> MGSSHHHHHHSQDPMEIPLSSGNVNTPDVRSSGILYINIYPIVNYPETIKVSAIPYYEEFLPGKWKKRIGDLIYLYGYGIENEFDEIDNSNALFGKIFRKYLLDILSENIATPWQLKELGSTLRLVKEITENYEFSNIIKLQYELIINVHHWQNTNFGIIVDLKINILDRENNQRISYTKIKDKYGESVKKKIWVSVQAFHRHLTPEGKKYATAMRDKFNLLTGLLKEAFGSSEDEKTFSTPDGEIKIVFKPLEIVEVSNNDGI

Here we focus on the prokaryotic Argonaute AfAgo from Archaeoglobus fulgidus DSM4304. Although phylogenetically classified as a long-B pAgo, AfAgo contains only MID and catalytically inactive PIWI domains, akin to short pAgos. We show that AfAgo forms a heterodimeric complex with a protein encoded upstream in the same operon, which is a structural equivalent of the N-L1-L2 domains of long pAgos. This complex, structurally equivalent to a long PAZ-less pAgo, outperforms standalone AfAgo in guide RNA-mediated target DNA binding.

Comparison of this 172 aa ORF to a homologous sequence found in a nearly identical AfAgo-encoding genetic island present in the genome of a related strain A. fulgidus DSM88774 revealed that it contains a premature STOP codon due to a 2 bp deletion. To study the structure and function of the full-length upstream protein, the restored full-length open reading frame, with the missing TA nucleotides inserted, was cloned into an E. coli expression vector and the corrected protein was subsequently purified by liquid chromatography. We were able to solve its structure by X-ray crystallography in two symmetry groups: P1 (resolution 1.85 Å) and P3221 (resolution 1.4 Å). Two full-length upstream protein chains found in the asymmetric unit of the P1 structure, and a single chain found in the asymmetric unit of the P3221 structure overlap with an RMSD of 0.85 Å (determined using PDBe Fold). We henceforth refer to the full-length upstream protein as AfAgo-N. The upstream protein (AfAgo-N) is the structural equivalent of the N-L1-L2 domains of long pAgo proteins.>[2x]MGSDKIHHHHHHMKAVRVHILGSGGREHAIGWAFAKQGYEVH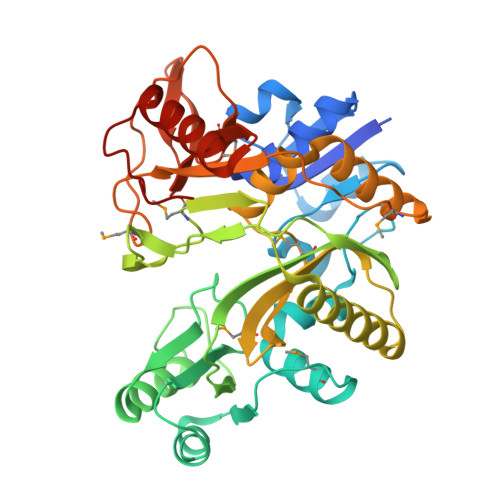FYPGNAGTKRDGTNHPYEGEKTLKAIPEEDIVIPGSEEFLVEGVSNWRSNVFGPVKEVARLEGSKVYAKRFMKKYGIRTARFEVAETPEELREKIKKFSPPYVIKADGLARGKGVLILDSKEETIEKGSKLIIGELIKGVKGPVVIDEFLAGNELSAMAVVNGRNFVILPFVRDYKRLMDGDRGPNTGGMGSWGPVEIPSDTIKKIEELFDKTLWGVEKEGYAYRGFLYLGLMLHDGDPYILEYNVRLGDPETEVIVTLNPEGFVNAVLEGYRGGKMEPVEPRGFAVDVVLAARGYPDAPEKGKEITLPEEGLIFFAGVAEKDGKLVTNGGRVLHCMGTGETKEEARRKAYELAEKVHFEGKTYRRDIAL>[2x]GMIKETVFKSFD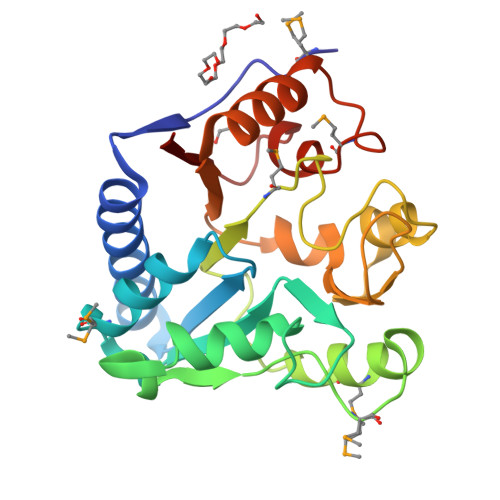TPSALEQQLASKIASQLQEAVDARGKASLVVSGGSTPLKLFQLLSMKSIDWSDVYITLADERWVEADADASNERLVREHLLQNRASNAKFRGLKNMFSTAEAGADMAAESLSNFPRPFDVVVLGMGNDGHTCSWFPCSAELENALTTQALCVATNPTTAPHGRITLSKSAILNSRQIYLHLVGEQKLSVYRQALESDDVHAMPIRAVLAQRKTPVDVFWSA> MAHHHHHHVGTGSNDDDDKSPDPPWELTILH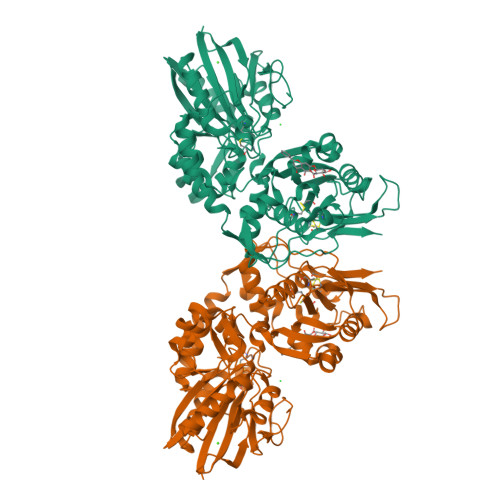TNDVHSRLEQTSEDSSKCVDASRCMGGVARLFTKVQQIRRAEPNVLLLDAGDQYQGTIWFTVYKGAEVAHFMNALRYDAMALGNHEFDNGVEGLIEPLLKEAKFPILSANISASGPLASQISGLYLPYKVLPVGDEVVGIVGYTSKETPFLSNPGTNLVFEDEITALQPEVDKLKTLNVNKIIALGHSGFEMDKLIAQKVRGVDVVVGGHSNTFLYTGNPPSKEVPAGKYPFIVTSDDGRKVPVVQAYAFGKYLGYLKIEFDERGNVISSHGNPILLDSSIPEDPSIKADINKWRIKLDDYSTQELGKTIVYLDGSSQSCRFRECNMGNLICDAMINNNLRHADEMFWNHVSMCILNGGGIRSPIDERNDGTITWENLAAVLPFGGTFDLVQLKGSTLKKAFEHSVHRYGQSTGEFLQVGGIHVVYDLSRKPGDRVVKLDVLCTSCRVPSYDPLKMDEVYKVILPNFLANGGDGFQMIKDELLRHDSGDQDINVVSTYISKMKVIYPAVEGRIKFS> GAMDIS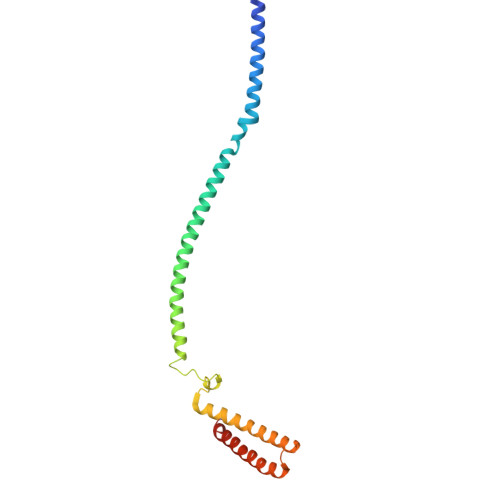PTNHHEMLQNLQTVVNELYREDVDYVADKILTRQTVMQESIARFHEIIAIDKNHLRAVEQAIEQTMHSLNAQIDVLTANRAKVQQFSSTSHVDDEDVNSIAVAKTDGLNQLYNLVAQDYALTDTIECLSRMLHRGTIPLDTFVKQGRELARQQFLVRWHIQRITSPLS>MAKEVIVYTSNTCPHCFTVKEFLSENNVEFTEKNIQTDAAARKELMKKGIMAVPVIQIDEEVVVGFDRDKIEEL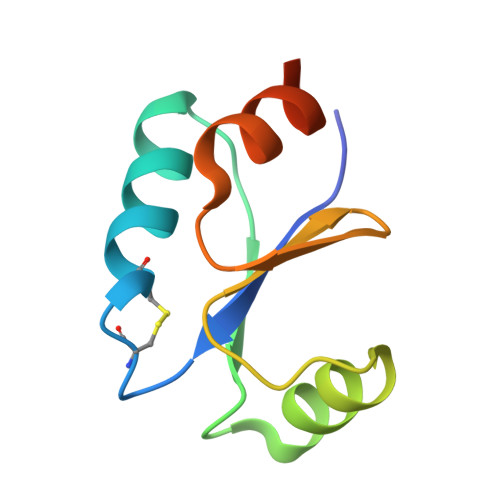LGLEHHHHHH[5x]>[4x]FNLPPGNYKKPVLLKSTETGQYLRINPDGEVDGTRDRSDVHIQFQISPEGNGEVLLKSTETGQYLRINPDGEVDGTRDRSDVHIQFQISPEGNGEVLLKS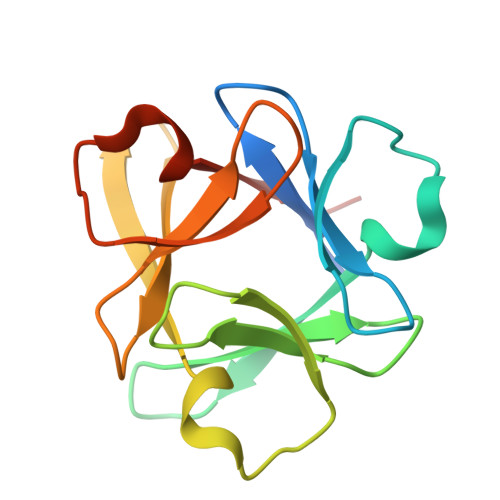TETGQYLRINPDGEVDGTRDRSDVHIQFQISPEGNG> MIDEPTGLYNRLRLQEDVSLRLQRDGALTVIAADLLPLALLNTIIRTLGYPFSNDLMLEARDRIRAELPDFTLY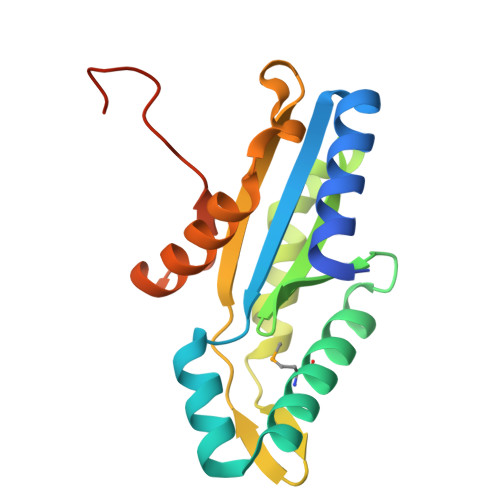KISPTRFGLLLPRQQQEETESVCLRLLRAFESPVVCRGIPIKANVGLGVLPLADDTLDGDQDWLRLVVSAADDARDRGVGWARYNPPLDQAQQRLEHHHHHH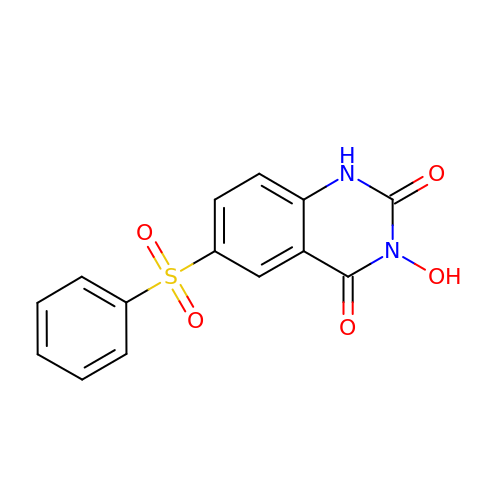3-hydroxy-6-(phenylsulfonyl)quinazoline-2,4(1H,3H)-dione | C14 H10 N2 O5 S | OWPKYKLZQGFBAE-UHFFFAOYSA-N>[2x]MGGSVIVIDSKAAWDAQLAKGKEEH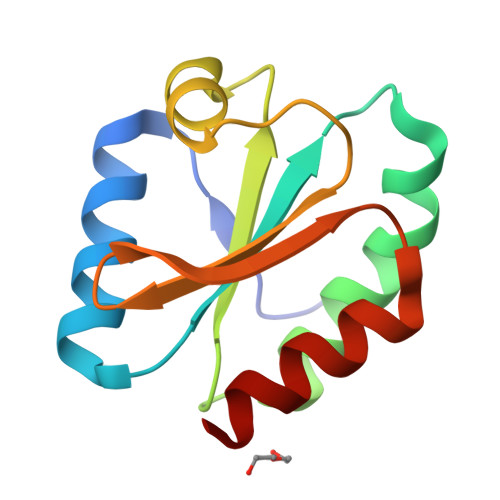KPIVVDFTATWSGPCKMIAPLFETLSNDYAGKVIFLKVDVDAVAAVAEAAGITAMPTFHVYKDGVKADDLVGASQDKLKALVAKHAAA>[4x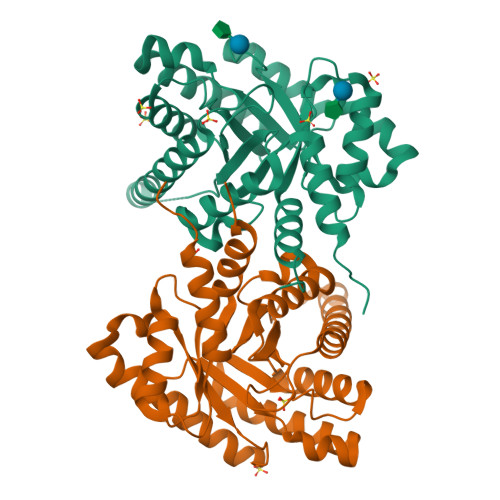]MGSSHHHHHHENLYFQGIYKQFTSRTLLNFFEVAALTDGETNESVAAVCKIAAKDPAIVGVSVRPAFVRFIRQELVKSAPEVAGIKVCAAVNFPEGTGTPDTVSLEAVGALKDGADEIECLIDWRRMNENVADGESRIRLLVSEVKKVVGPKTLKVVLSGGELQGGDIISRAAVAALEGGADFLQTSSGLGATHATMFTVHLISIALREYMVRENERIRVEGINREGAAVRCIGIKIEVGDVHMAETADFLMQMIFENGPRSIVRDKFRVGGGFNLLKELRDCYESWDSVGVS> GSASPTPPYLKWAESLHSLLDDQDGISLFRTFLKQEGCADLLDFWFACTG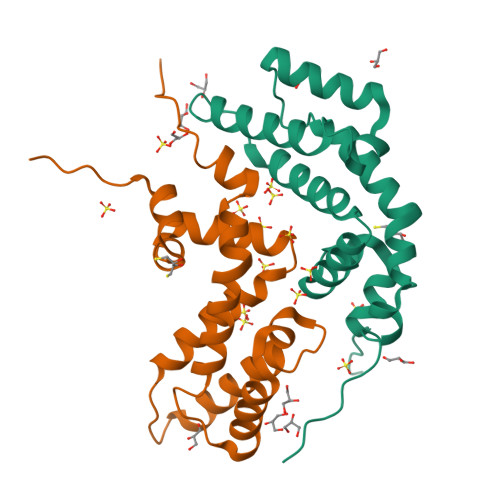FRKLEPCDSNEEKRLKLARAIYRKYILDNNGIVSRQTKPATKSFIKGCIMKQLIDPAMFDQAQTEIQATMEENTYPSFLKSDIYLEYTRTGSESPKV>MGHHHHHHHHHHSSGHGTIQGSEDLYFQSHMMALVDLVRAGGYSVEYPQFSSMAKLKAFPHSEDGQLVRLLSWHEGVGLGGGLFKVSTSSTATGNDGTVVVASNGVRLLRVVNGPIWADMFGALPNSDIDSMPAVAAAYAYAASVNTDLYIGVATYKFKGSTPINVDPSRAGIIGYQGKVRIDCSEFTGSIVFSINSSYSYTPAAYYNNLSPALQGLYVFGAKTSGVDGLLVGRETVGSDKSYNGQTEVRECTFDKFDRNIRMGHNSWRFVFYKVNSLNALSPNGILYVPAGLDDSGEILSFYHCQFFDGAGSNIRLSCSSYTMVFNTCSFLNITFFVDSASSATVTCNGCNFANPGSASTRRYVDISAGHTNVFNIIGGSIVTNSNPGQTQALLYVSTDNLLNLVGVTAPYGGHYQQEQELGYHAFIGGAGTVTTSGVMLQLRNGAGTCPLHSSLSTFSNWNFGYGNLNAWTVDKGTGTSSVVEYLANAGPKGTEGAMRVAPVSVGTNVSQVQAVTN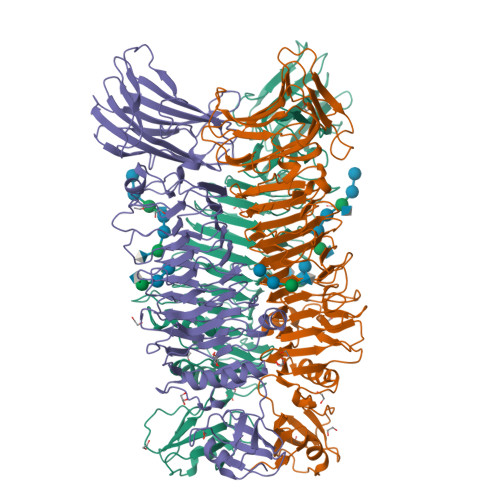PGMFSMSCMVNIATTPGNAGQVSIGFLDAAGNSLPGGVSANLGTTTGWQVIGKNTLRGKVPIGAKQVRVNIQTVAGADVKYAYLLCNVVKKLGC[3x]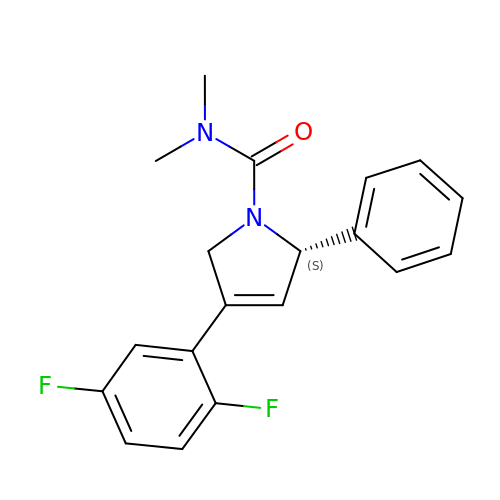(2S)-4-(2,5-DIFLUOROPHENYL)-N,N-DIMETHYL-2-PHENYL-2,5-DIHYDRO-1H-PYRROLE-1-CARBOXAMIDE | C19 H18 F2 N2 O | WFFMEXQHWXEKBV-SFHVURJKSA-N> SNIQTGAERMPHDLSHLGFLAGQIGRLITISTTPVIAGDSFEMDAVGALRLSPLRRGLAIDSTVDIFTFYVPHRHVYGEQWIKFMKDGVNATPLPTVNTTGYIDHAAFLGTINPDTNKIPKHLFQGYLNIYNNYFKAPWMPDRTEANPNELNQDDARYGFRCCHLKNIWTAPLPPETELSRQMTTSTTSIDIMGLQAAYANLHTDQERDYFMQRYRDVISSFGGKTSYDADNRPLLVMRSNLWASGYDVDGTDQTSLGQFSGRVQQTYKHSVPRFFVPEHGTMFTLALVRFPPTATKEIQYLNAKGALTYTDIAGDPVLYGNLPPREISMKDVFRSGDSSKKFKIAEGQWYRYAPSYVSPAYHLLEGFPFIQEPPSGDLQERVLIRHHDYDQCFQSVQLLQWNSQVKFNVTVYRNLPTTRDSIMTS;> MFQTFISRHNSNFFSDKLVLTSVTPASS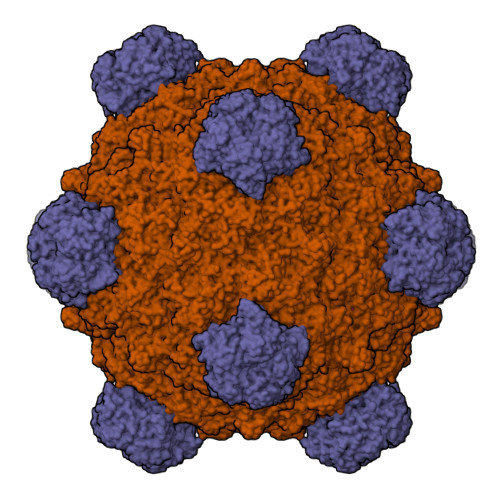APVLQTPKATSSTLYFDSLTVNAGNGGFLHCIQMDTSVNAANQVVSVGADIAFDADPKFFACLVRFESSSVPTTLPTAYDVYPLNGRHDGGYYTVKDCVTIDVLPRTPGNNVYVGFMVWSNFTATKCRGLVSLNQVIKEIICLQPLK;> SKGKKRSGARPGRPQPLRGTKGKRKGARLWYVGGQQF> PICTNCCAG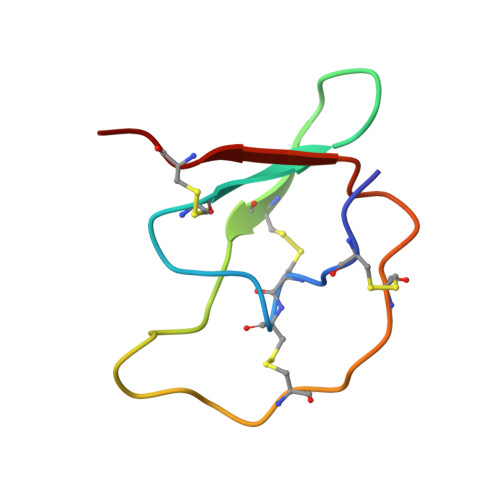YKGCNYYSANGAFICEGQSDPKKPKACPLNCDPHIAYSKCPR(2~{R})-2-[[4-[[4-methoxy-2-(trifluoromethyl)phenyl]methylcarbamoyl]phenyl]methyl]butanoic 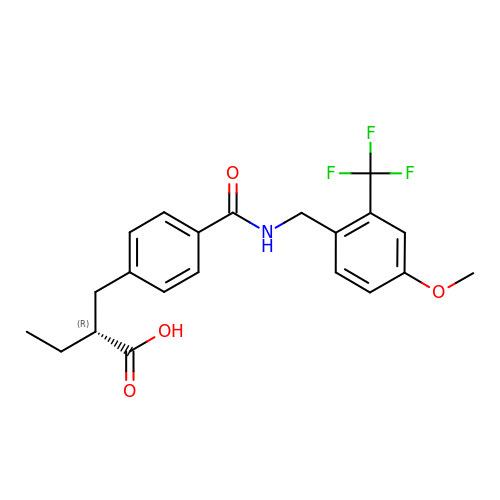acid | C21 H22 F3 N O4 | VPAHYLNIDWFBPW-CQSZACIVSA-N> DITVYNGQHKEAATAVAKAFEQETGIKVTLNSGKSEQLAGQLKEEGDKTPADVFYTELTATFADLSEAGLLAPISEQTIQQTAQKGVPLAPKKDWIALSGRSRVVVYDHTKLSEKDMEKSVLDYATPKWKGKIGYVST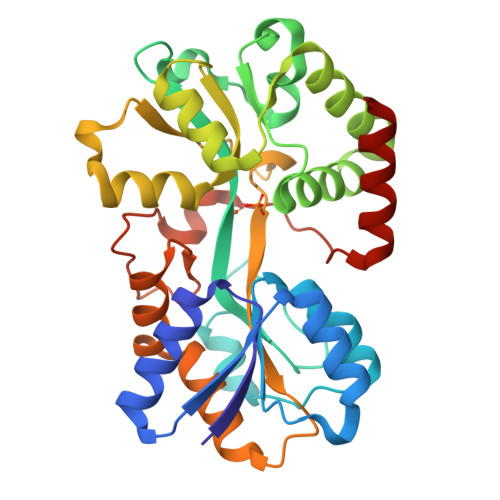SGAFLEQVVALSKMKGDKVALNWLKGLKENGKLYAKNSVALQAVENGEVPAALINNYYWYNLAKEKGVENLKSRLYFVRHQDPGALVSYSGAAVLKASKNQAEAQKFVDFLASKKGQEALVAARAEYPLRADVVSPFNLEPYEKLEAPVVSATTAQDKEHAIKLIEEAGLK Although first discovered as a placental antigen present in the circulation during human pregnancy, the metzincin metalloproteinase PAPP-A (pregnancy-associated plasma protein-A, pappalysin-1, EC 3.4.24.79) is ubiquitously expressed in human tissues. PAPP-A is able to cleave insulin-like growth factor binding proteins (IGFBP) -2, -4, and -5 in the extracellular environment. It consequently causes the release of bound bioactive IGF-1 or -2, which are potent growth factors. The paralogue proteins stanniocalcin (STC)-1 and -2 were recently identified as potent endogenous PAPP-A inhibitors and thus connected with the IGF system.

We have determined the structure of the metalloproteinase, PAPP-A, in complex with its endogenous inhibitor, STC2, to a resolution of 3.1 Å. The highest resolution (3.1 Å) was obtained for the STC2 subunit and the N-terminal approximately 1000 residues of the PAPP-A subunit. Some regions, in particular some of the SCR domains (4–7 Å) and M5-M6 (5–8 Å), were determined to a lower resolution, and will benefit from further structural analysis. (3) C120 of STC2, which is required for the function of STC2 in vivo, connects specifically to C732 of the M2 domain of PAPP-A, thus preventing dissociation of the complex. (2) Structural and biochemical data show that STC2 binds to the PAPP-A C domain, and that removal of Ca2+ from LNR3 diminishes its binding. While the core of the CD is similar in structure to other metzincins, in particular the two known unicellular pappalysin structures, the PAPP-A CD stands out in several regards, most notable by the inserted LNR modules. In PAPP-A, the LNR modules do not appear to have a similar role, but rather interact with either substrate or inhibitor. The pappalysin S1′ specificity pocket has a conserved aspartate in its bottom (D641 of PAPP-A)13,39 to accommodate the basic side chain of the substrate residue on the C-terminal side of the scissile bond, the P1′ position. Thus, the C612-C643 disulfide bond, which connects the ZnM loop (V573-F635) underneath the active site cleft to the CD core, may be important for keeping D641 in a position to provide specificity. Although the inhibited complex cannot cleave IGFBP-4, the PAPP-A active site is accessible and active toward a synthetic peptide derived from IGFBP-4.

>[2x]EARGATEEPSPPSRALYFSGRGEQLRLRADLELPRDAFTLQVWLRAEGGQRSPAVITGLYDKCSYISRDRGWVVGIHTISDQDNKDPRYFFSLKTDRARQVTTINAHRSYLPGQWVYLAATYDGQFMKLYVNGAQVATSGEQVGGIFSPLTQKCKVLMLGGSALNHNYRGYIEHFSLWKVARTQREILSDMETHGAHTALPQLLLQENWDNVKHAWSPMKDGSSPKVEFSNAHGFLLDTSLEPPLCGQTLCDNTEVIASYNQLSSFRQPKVVRYRVVNLYEDDHKNPTVTREQVDFQHHQLAEAFKQYNISWELDVLEVSNSSLRRRLILANCDISKIGDENCDPECNHTLTGHDGGDCRHLRHPAFVKKQHNGVCDMDCNYERFNFDGGECCDPEITNVTQTCFDPDSPHRAYLDVNELKNILKLDGSTHLNIFFAKSSEEELAGVATWPWDKEALMHLGGIVLNPSFYGMPGHTHTMIHQIGHSLGLYHVFRGISEIQSCSDPCMETEPSFETGDLCNDTNPAPKHKSCGDPGPGNDTCGFHSFFNTPYNNFMSYADDDCTDSFTPNQVARMHCYLDLVYQGWQPSRKPAPVALAPQVLGHTTDSVTLEWFPPIDGHFFERELGSACHLCLEGRILVQYASNASSPMPCSPSGHWSPREAEGHPDVEQPCKSSVRTWSPNSAVNPHTVPPACPEPQGCYLELEFLYPLVPESLTIWVTFVSTDWDSSGAVNDIKLLAVSGKNISLGPQNVFCDVPLTIRLWDVGEEVYGIQIYTLDEHLEIDAAMLTSTADTPLCLQCKPLKYKVVRDPPLQMDVASILHLNRKFVDMDLNLGSVYQYWVITISGTEESEPSPAVTYIHGSGYCGDGIIQKDQGEQCDDMNKINGDGCSLFCRQEVSFNCIDEPSRCYFHDGDGVCEEFEQKTSIKDCGVYTPQGFLDQWASNASVSHQDQQCPGWVIIGQPAASQVCRTKVIDLSEGISQHAWYPCTISYPYSQLAQTTFWLRAYFSQPMVAAAVIVHLVTDGTYYGDQKQETISVQLLDTKDQSHDLGLHVLSCRNNPLIIPVVHDLSQPFYHSQAVRVSFSSPLVAISGVALRSFDNFDPVTLSSCQRGETYSPAEQSCVHFACEKTDCPELAVENASLNCSSSDRYHGAQCTVSCRTGYVLQIRRDDELIKSQTGPSVTVTCTEGKWNKQVACEPVDCSIPDHHQVYAASFSCPEGTTFGSQCSFQCRHPAQLKGNNSLLTCMEDGLWSFPEALCELMCLAPPPVPNADLQTARCRENKHKVGSFCKYKCKPGYHVPGSSRKSKKRAFKTQCTQDGSWQEGACVPVTCDPPPPKFHGLYQCTNGFQFNSECRIKCEDSDASQGLGSNVIHCRKDGTWNGSFHVCQEMQGQCSVPNELNSNLKLQCPDGYAIGSECATSCLDHNSESIILPMNVTVRDIPHWLNPTRVERVVCTAGLKWYPHPALIHCVKGCEPFMGDNYCDAINNRAFCNYDGGDCCTSTVKTKKVTPFPMSCDLQGDCACRDPQAQEHS;> RLSLQNTAEIQHCLVNAGDVGCGVFECFENNSCEIRGLHGICMTFLHNAGKFDAQGKSFIKDALKCKAHALRHRFGCISRKCPAIREMVSQLQRECYLKHDLCAAAQENTRVIVEMIHFKDLLLHEPYVDLVNLLLTCGEEVKEAITHSVQVQCEQNWGSLCSILSF> TSDPV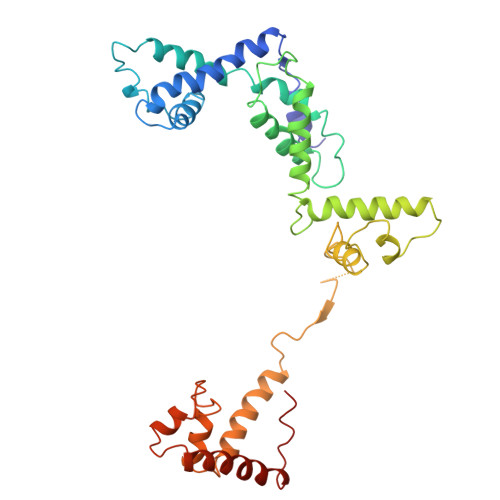RQYLHEIGQVPLLTLEEEIDLARKVEEGMEAIKKLSEATGLDQELIREVVRAKILGTARVEEVDGKLKSLPKELKRYLHIAREGEAARQHLIEANLRLVVSIAKKYTGRGLSFLDLIQEGNQGLIRAVEKFEYKRRFKFSTYATWWIRQAINRAIADQARTIRIPVHMVETINKLSRTARQLQQELGREPSYEEIAEAMGPGWDAKRVEETLKIAQEPVSLETPIGDEKDSFYGDFIPDENLPSPVEAAAQSLLSEELEKALSKLSEREAMVLKLRKGLIDGREHTLEEVGAYFGVTRERIRQIENKALRKLKYHESRTRKLRDFLE>EAKKEIPLKYGATNEGKRQDPAMQKFRDNRLGAFIHWGLYAIPGGEWNGKVYGGAAEWLKSWAKVPADEWLKLMDQWNPTKFDAKKWAKMAKEMGTKYVKITTKHHEGFCLWPSKYTKYTVANTPYKRDILGELVKAYNDEGIDVHFYFSVMDWSNPDYRYDIKSKEDSIAFSRFLEFTDNQLKELATRYPTVKDFWFDGTWDASVKKNGWWTAHAEQMLKELVPGVAINSRLRADDKGKRHFDSNGRLMGDYESGYERRLPDPVKDLKVTQWDWEACMTIPENQWGYHKDWSLSYVKTPIEVIDRIVHAVSMGGNMVVNFGPQADGDFRPEEKAMATAIGKWMNRYGKAVYACDYAGFEKQDWGYYTRGKNDEVYMVVFNQPYSERLIVKTPKGITVEKATLLTTGEDITVVETTRNEYNVSVPKKNPGEPYVIQLKVRAAK[2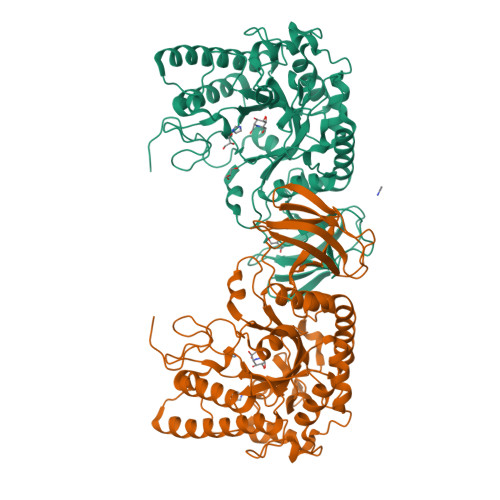x]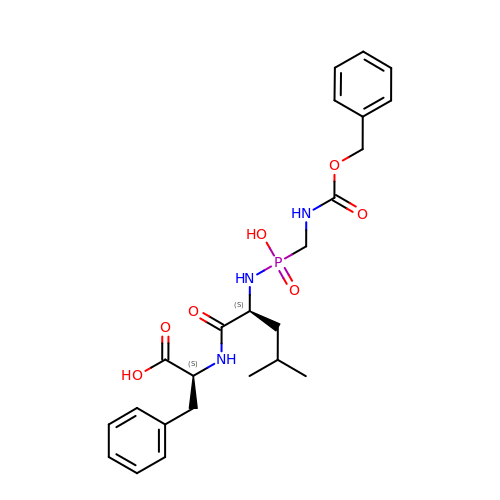N-[(R)-({[(benzyloxy)carbonyl]amino}methyl)(hydroxy)phosphoryl]-L-leucyl-L-phenylalanine | C24 H32 N3 O7 P | LSBJYKCMZGPGPG-SFTDATJTSA-N> HKDDQLICVNENGGCEQYCSDHTGTKRSCRCHEGYSLL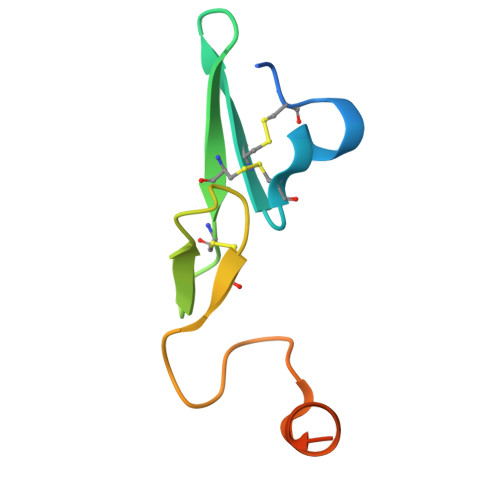ADGVSCTPTVEYPCGKIPILEKRNASKPQGR> MEVARGLEGVLFTESRMCYIDGQQGKLYYYGI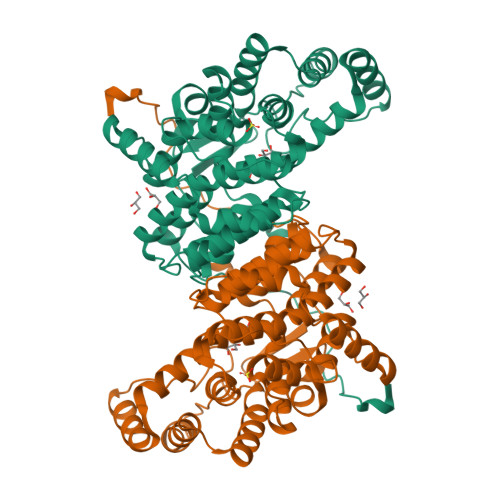PIQELAEKSSFEETTFLLLHGRLPRRQELEEFSAALARRRALPAHLLESFKRYPVSAHPMSFLRTAVSEFGMLDPTEGDISREALYEKGLDLIAKFATIVAANKRLKEGKEPIPPREDLSHAANFLYMANGVEPSPEQARLMDAALILHAEHGFNASTFTAIAAFSTETDLYSAITAAVASLKGPRHGGANEAVMRMIQEIGTPERAREWVREKLAKKERIMGMGHRVYKAFDPRAGVLEKLARLVAEKHGHSKEYQILKIVEEEAGKVLNPRGIYPNVDFYSGVVYSDLGFSLEFFTPIFAVARISGWVGHILEYQELDNRLLRPGAKYVGELDVPYVPLEARE>[2x]SGRFDQYPTKKGDFAIDGYLLDYSSPKQGCWVDGITVYGDIYIGKQNW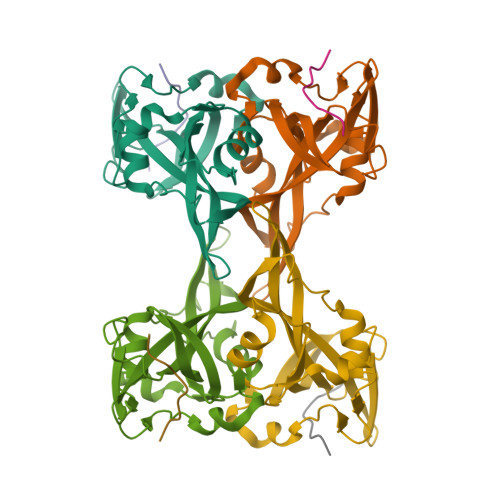GTYTRPVFAYLQYVETISGSGTFVIYQVVLVYAHNATSAGRQNANAFAYSKTQAVGSRVDLYYLSAITQRKRVIVPSSNAVTPLDWDTVQRNVLMENYNPGSNSGHFSFDWSAYNDPHRRY;>QPQSHSIELDEVSKEAASTRAALTSNL[2x]>[2x]LPNITILATGGTIAGGGDSATKSNYTAGKVGVENLVNAVPQLKDIANVKGEQVVNIGSQDMNDDVWLTLAKKINTDCDKTDGFVITHGTDTMEETAYFLDLTVKCDKPVVMVGAMRPSTSMSADGPFNLYNAVVTAADKASANRGVLVVMNDTVLDGRDVTKTNTTDVATFKSVNYGPLGYIHNGKIDYQRTPARKHTSDTPFDVS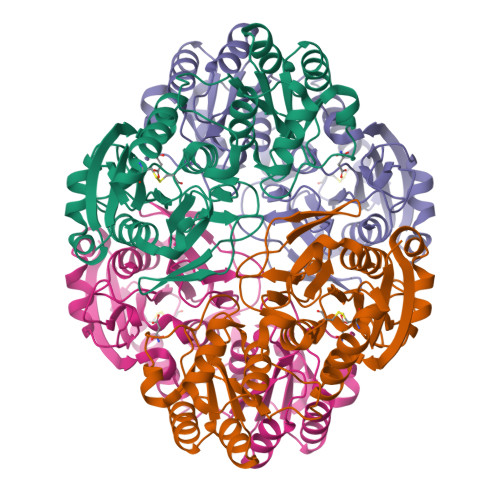KLNELPKVGIVYNYANASDLPAKALVDAGYDGIVSAGVGNGNLYKTVFDTLATAAKNGTAVVRSSRVPTGATTQDAEVDDAKYGFVASGTLNPQKARVLLQLALTQTKDPQQIQQIFNQY> MQEKSITIATEGGYAPWNFSGPGGKLDGFEIDLANALCEKMKAKCQIVAQNWDGIMPSLTGKKYDAIMAAMSVTPKRQEVIGFSIPYAAGINGFAVMGDSKLAEMPGLGETYSLDSQADAAKKAIADISSFLNGTTVGVQGSTTASTFLDKYFKGSVDIKEYKSVEEHNLDLTSGRLDAVLANATVLAAAIEKPEMKGAKLVGPLFSGGEFGVVAVGLRKEDTALKADFDAAIKAASEDGTIKTLSLKWFKVDVTPQHHHHHH

Two Agrobacterium ABC-transporters and their cognate periplasmic binding proteins (PBPs) OccJ and NocT import octopine and nopaline/octopine, respectively. Recognition and import of opines are conferred by periplasmic binding proteins (PBPs) and their associated ATP-binding cassette (ABC) transporters. The PBP OccJ is associated with the octopine transporter of octopine-type A. tumefaciens while NocT is associated with nopaline uptake in the nopaline-type A. tumefaciens. OccJ shares 47% sequence identity with NocT and belongs to cluster F within the PBP structural classification.

We report the X-ray structures of the unliganded PBP OccJ and its complex with octopine as well as a structural comparison with NocT and the related PBP LAO from Salmonella enterica, which binds amino acids (lysine, arginine and ornithine). The mature PBP OccJ (256 aa without the signal peptide) expression plasmid was obtained by cloning the occJ gene lacking the first twenty residues of the signal sequence that serves for localization to bacterial periplasm. The X-ray structures of the unliganded and liganded OccJ with octopine were solved at 2.35 and 2 Å resolution respectively. The liganded form adopts a closed conformation whereas the unliganded form adopts an open conformation. Indeed, superposition of the two structures results in an average RMSD of 4 Å for all Cα atoms and a structural comparison shows a 49° rotation around the hinge region of the C-terminal domain (residues 112–226) upon ligand binding once the N-terminal domains (residues 21–107 and 234–276) were superimposed leading to a movement of 10 Å for Thr163.(2R)-7-amino-2-(selanylmethyl)heptanoic 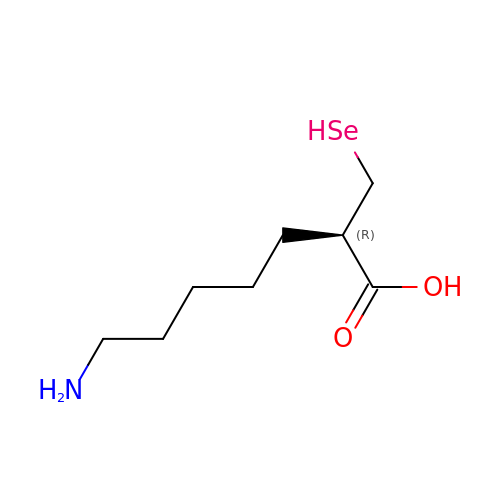acid | C8 H17 N O2 Se | PKYDFIWWGOFUJY-ZETCQYMHSA-N2,5-dimethyl-6-quinolin-4-yl-3~{H}-quinazolin-4-one 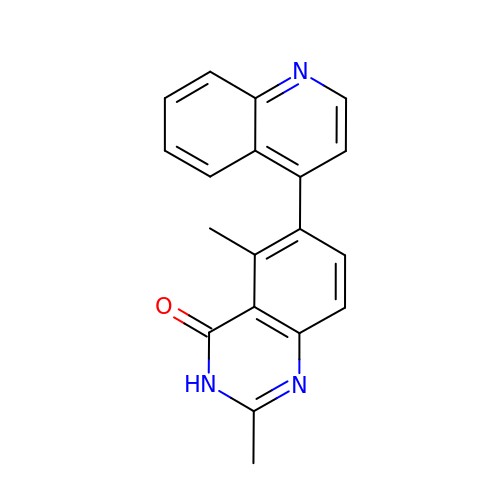| C19 H15 N3 O | CNEUJSQUCXSRDD-UHFFFAOYSA-N> SDMPVERILEAELAVEPKTETYVEANMGLNPSSPNDPVTNICQAADKQLFTLVEWAKRIPHFSELPLDDQVILLRAGWN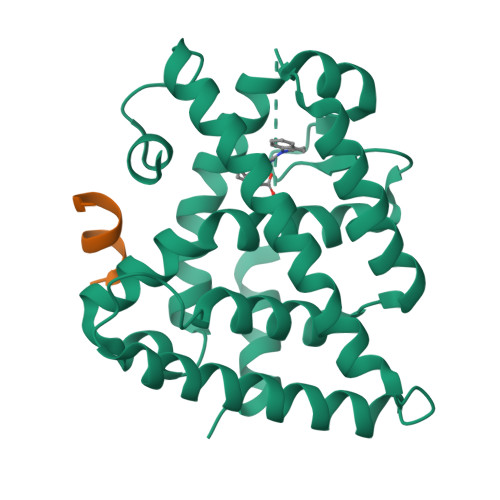ELLIASFSHRSIAVKDGILLATGLHVHRNSAHSAGVGAIFDRVLTELVSKMRDMQMDKTELGCLRAIVLFNPDSKGLSNPAEVEALREKVYASLEAYCKHKYPEQPGRFAKLLLRLPALRSIGLKCLEHLFFFKLIGDTPIDTFLMEMLEAPHQMT;> HSSLTERHKILHRLLQEGSPS1,3-dihydroxypropan-2-yl dodecanoate 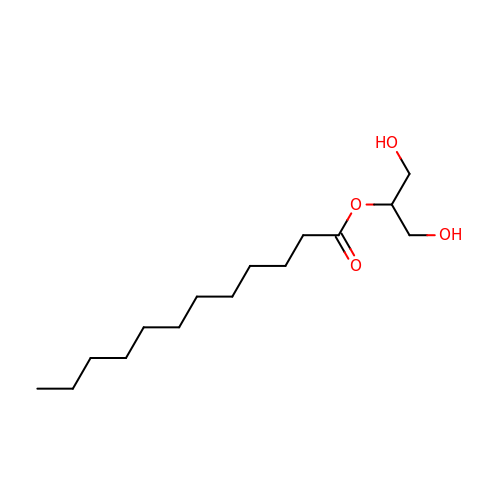| C15 H30 O4 | ZUCMOZYYSZYRRM-UHFFFAOYSA-N> MSARISLFAVVVED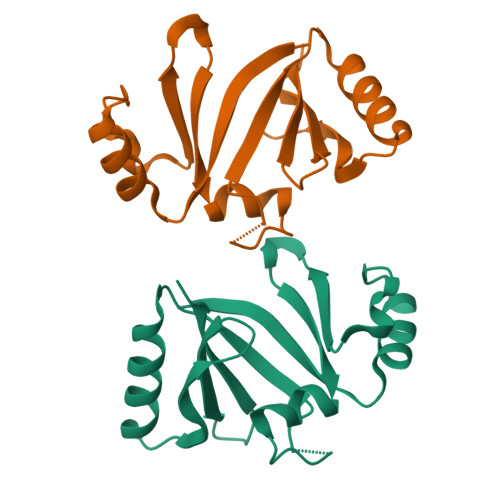MAKSLEFYRKLGVEIPAEADSAPHTEAVLDGGIRLAWDTVETVRSYDPEWQAPTGGHRFAIAFEFPDTASVDKKYAELVDAGYEGHLKPWNAVWGQRYAIVKDPDGNVVDLFAPLP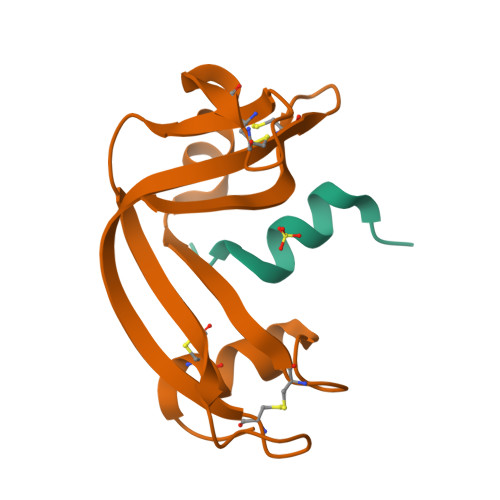> SSSNYCNQMMKSRNLTKDRCKPVNTFVHESLADVQAVCSQKNVACKNGQTNCYQSYSTMSITDCRETGSSKYPNCAYKTTQANKHIIVACEGNPYVPVHFDASV;> KETAAAKFERQHVDSX> MEGCVSNLMVCNLAYSGKLEELKESILADKSLATRTDQDSRTALHWACSAGHTEIVEFLLQLGVPVNDKDDAGWSPLHIAASAGRDEIVKALLGKGAQVNAVNQNGCTP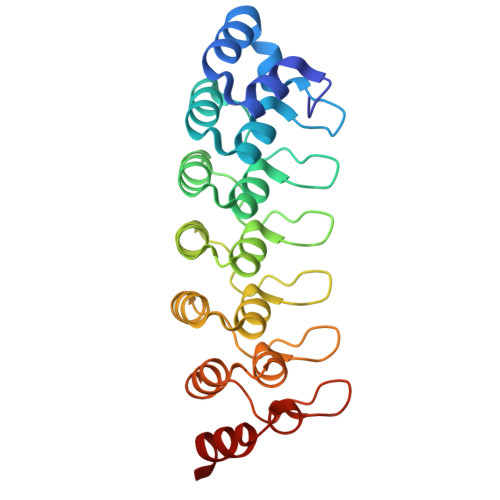LHYAASKNRHEIAVMLLEGGANPDAKDHYEATAMHRAAAKGNLKMIHILLYYKASTNIQDTEGNTPLHLACDEERVEEAKLLVSQGASIYIENKEEKTPLQVAKGGLGLILKRMVEG> ITLKVAIYPYVPDPARFQAAVLDQWQRQEPGVKLEFTDWDSYSADPPDDLDVFVLDSIFLSHFVDAGYLLPFGSQDIDQAEDVLPFALQGAKRNGEVYGLPQILCTNLLFYRKGDLKIGQVDNIYELYKKIGTSHSEQIPPPQNKGLLINMAGGTTKASMYLEALIDVTGQYTEYDLLPPLDP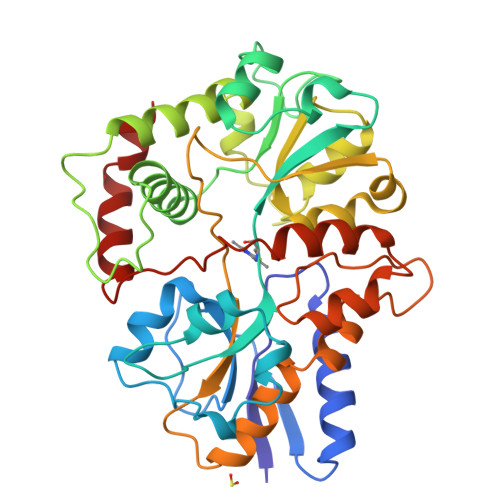LNDKVIRGLRLLINMAGEKPSQYVPEDGDAYVRASWFAQGSGRAFIGYSESMMRMGDYAEQVRFKPISSSAGQDIPLFYSDVVSVNSKTAHPELAKKLANVMASADTVEQALRPQADGQYPQYLLPARHQVYEALMQDYPIYSELAQIVNKPSNRVFRLGPEVRTWLKDAKQVLPEALG>MAHHH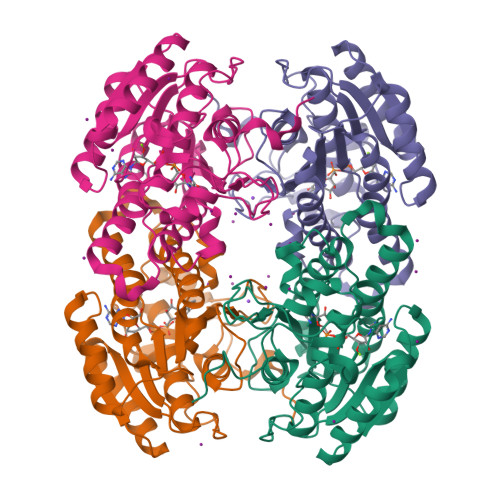HHHMAVDAPPAAQGLTNPVDLYPKPPFPHQVQAPPGLASRMQPRPDHGEQSYRGRGRLVGRKTLVTGGDSGIGRAAAIAFAREGADVAIGYLPVEESDAREVVALIRAAGRQAVALPGDIRDETFCQRLVARAAEALGGLDILVNNAARQQALDSIGEMTTEHFDATVKTNLYGMFWITKAAIPHLPPGASIINTTSVQAVRASANLLDYATTKAGIIAFTRSLAKQLGPRGIRVNAVAPGPYWTPLQSSGGQPPETVVNYAAGSPYGRPGQPAEIAPLYVALAASETSYANGQVWGADGGLGIF[8x]> 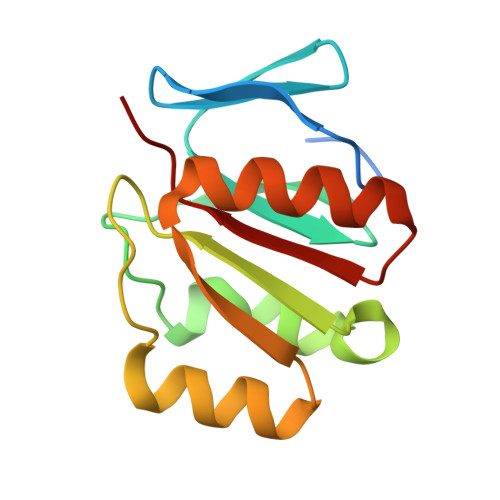MSHAIQIREAHFPGRAPIDAYGNGGFRFADMSHRGSIICIPSGIYGIDMTGPVPTQEDISRVLEESDQIEVLLIGTGVELLRLPEELRVLLWEKRISSDTMSTGAAVRTFNVLLAEDRAVAALLFAVE>[3x]SNAMLDNRPIGVFDSGIGGLTIVKNLMSILPNEDIIYFGDIARIPYGTKSRATIQKFAAQTAKFLIDQEVKAIIIACNT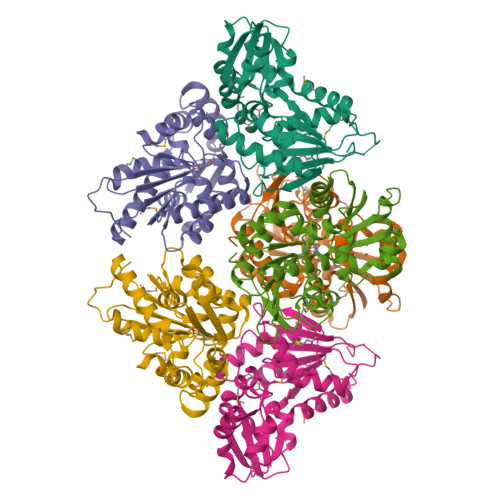ISAIAKDIVQEIAKAIPVIDVITAGVSLVDNLNTVGVIATPATINSNAYALQIHKKNPNIEVYSNPCGLFVSMIEEGFVSGHIVELVAKEYLSYFHDKNIQALILGCTHYPIIKESIAKILDVKLIDPSLQASKMLYSLLFENKLLNTTKSNPEYRFYVTDIPLKFRSVGEMFLQTEMQHLEIVSLDSY>MGHHHHHHGMTLSAKQQSALLLLGWLQLQYGHPDRARILLDALLALHPEHKEGRRALVVSLLKLQKGSMAKEHCTLLQEQGEQSAALWLCVSRACQQEGNLEEARSAYQRYLAQGALL[2x];>[2x]GAMERLADRALLDFATPHRGFHDLLRPVDFHQAMQGLRSVLAEGQSPELRAAAILLEQMHADEQLMQMTLHLLHKV

SctX proteins are secreted substrates and are essential components of type III secretion systems. The dedicated chaperone SctY escorts SctX proteins to the secretion machinery, where the hydrophobic helix at the C-terminus of SctX mediates recognition by the export apparatus. The type III secretion substrate SctX binds its chaperone at two distinct sites: (i) its α1 helix interacts with the concave groove of SctY and (ii) the two C-terminal helices α2 and α3 cover the large hydrophobic surface formed by the N-terminal TPR of the chaperone.

We were unable to express A. hydrophila His6-AscY in E. coli, but were able to solubly co-express AscX with P. luminescens subsp. laumondii His6-LscY. The AscX49–LscY complex was reductively methylated to enable crystallization and diffracted to approximately 2 Å resolution. The asymmetric unit contains two heterodimers related via a tNCS vector (0.000, 0.500, 0.500) with a height of 83% compared with the origin Patterson peak. The two AscX49–LscYmeth dimers in the asymmetric unit are virtually identical and both exhibit the α3 bend in the substrate as described for AscX31–YscY. Notably, the bend occurs at the same residue, Ala106. While the C-terminal end of the α2 helix superimposes well between the two complexes, the N-terminal end is rotated by about 13°, resulting in a shift of about 6.1 Å of His76 at the N-terminal end of the helix. Furthermore, the α3 helix appears to be rotated by about 10° in a similar fashion, with Ala106 being displaced by approximately 5.6 Å. A possible explanation for this shift is the presence of Phe12 in YscY instead of Ala10 in LscY, which causes steric conflicts with Met79 in the α2 helix of AscX. An exchange of Phe12 in YscY to Ala10 in LscY and AscY allows the repositioning of SctX helices α2 and α3.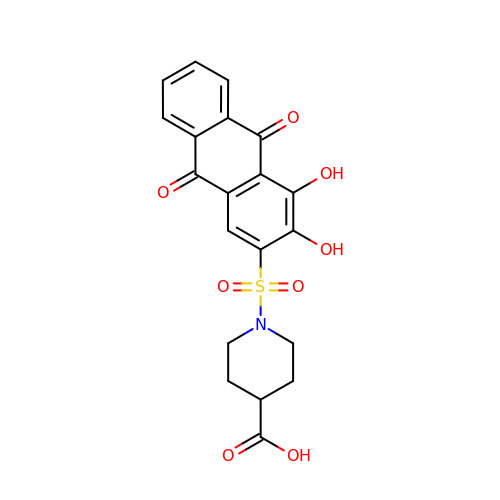1-(3,4-dihydroxy-9,10-dioxo-9,10-dihydroanthracene-2-sulfonyl)piperidine-4-carboxylic acid | C20 H17 N O8 S | GAZMUVGYYAVFHP-UHFFFAOYSA-N> NPRAQVFEYFKLKVPATRGAVLKAHINHLGNVAAMVSFILVHHLSWDPATQGVLWAPATMFYARLYQLGLDAVALSPDALFVARMHLLAAIILWGFGHVKSPAEEKFLEKVTMGKALVAQFHFFALIATLWGLHMAFYGILGPSGKLEPTGLSFDM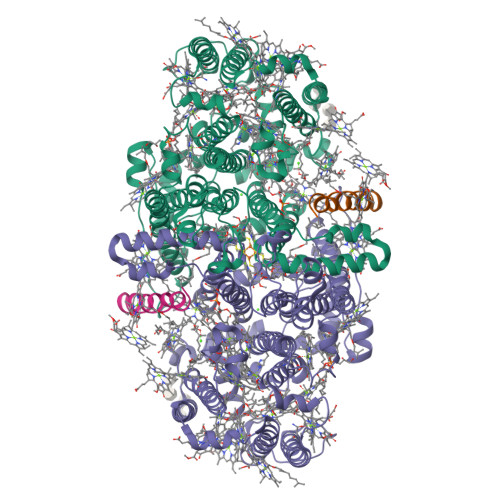FGPITPATMAGNHVAFGAVFFLGGIFHYFAGFNTKRFAFFEKDWEAVLSVSCQILAFHFATVVFAMIIWQHPQLGFGFMREYAVSQYAGPELKMIAQSNPGLLVKQAILGHLVMGIMFWIGGVFHGAHFMLRVLNDPKLAEEMKDFKFIKRCYDHEFQKKFLALIMFGAFLPIFVSYGIATHNTIADIHAASKTGLFAHMTYINIGTPLHDAIFGSKGSISEFVAAHAIAGGLHFTMVPMWRMVFFSKVSPWTTKVGMKAKRDGEFPCLGPAYGGTCSISLVDQFYLAIFFSLQVIAPAWFYIDGCWMGSFVAVAAPYNDIYQAALATFNSHNPLHQLSPLTNMGYFSYIIQQTTAMFSRYDGHMIQALLGAHFIWAFTFSMLFQYRGSRDEGAMVLKWAHQQVGVGFAGKMYNRALSLKEGKAIGCFLFFKMTIVCMWALAMV;> YSPTFNVAHILAFFFLFLHIPFYFV> RRHVLLQAEFYQRSEGPDKAWAQFGFHFDADELFHVELDAAQTVWRLPEFGRFASFEAQGALQNMAVGKQNLEVMISNSNRSQQDFVTPELALFPAEAVSLEEPNVLICYADKFWPPVATMEWRRNGAVVSEGVYDSVYYGRPDLLFRKFSYLPFVPQRGDVYSCAVRHWGAEGPVQR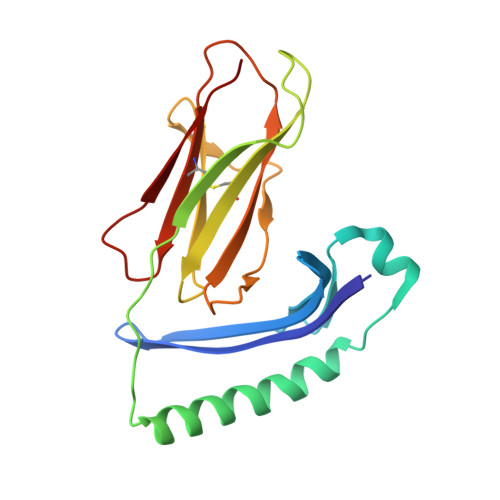MWEPE> SNAMNKEQLQQMRQAPGFVGALDQSGGSTPKALKAYGIQPDAYQSEEEMFDLIHQMRTRMITSPAFATGKIIGVILFERTMRGKIEGMPTADFLWEKRHIVPFLKVDKGLQDEANGVQLMKPFPELGKLCEEAVGYHVFGTKMRSVIKQANEQGIRDIVEQQFQWGKEILSHGLVPILEPEVDIHCPEK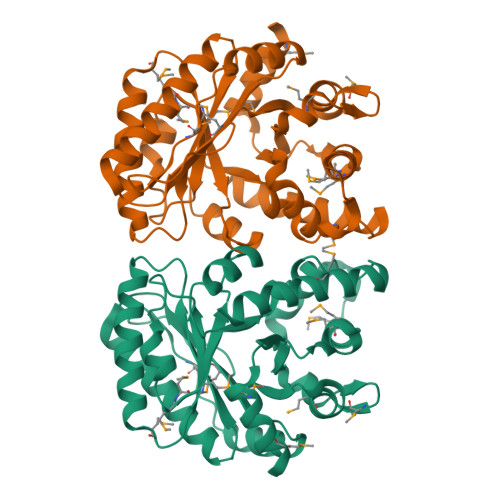AKAEEILKRELLAQLDKMTEPVMLKITIPTVDNFYKEIIEHPMMLRVVALSGGYSREQANELLSRNHGVIASFSRALVEGLSARQTDAEFNAMLEASIEDVYQASIK> VHFKDGVYENIPFK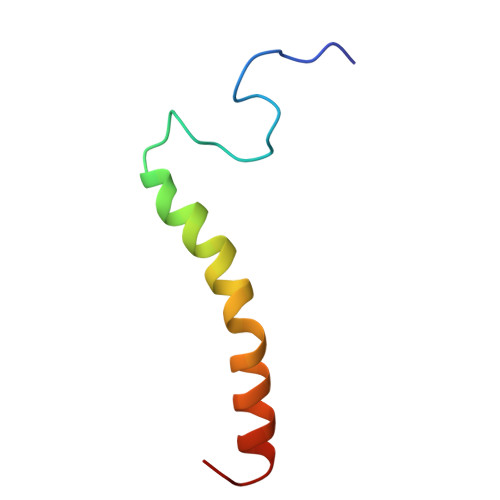VKGRKTPYALSHFGFFAIGFAVPFVACYVQLKKSGAF>HHHHHHMTALTLPED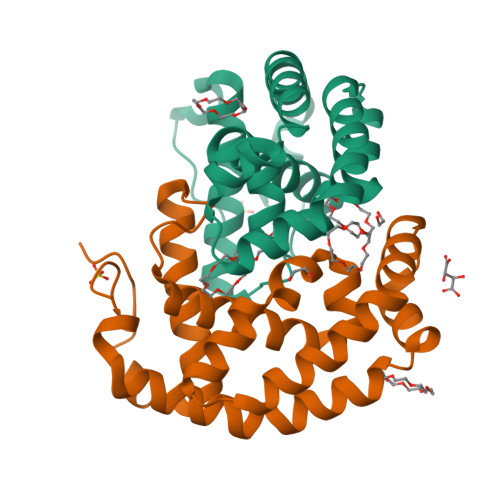IRQQEPSALLYTLVSAYLEHTAQTGDESLSCLSDDQHTLTAFCYLDSQVEEGGFVQLIASGYGEYIFRNPLADSLRRWKIKAVPKVLDKAKALYEQHGKTIETLADGGADIPSLRKQFPEFEEWDGAYYEAAEQDLPLLAEHIQSNWETFAHIGQA[2x]>GSHMGKAAIGGPFSLIRDDGKRVTEKNLMGKWTILYFGFTHCPDICPDELIKLAAAIDKIKENSGVDVVPVFISVDPERDTVQQVHEYVKEFHPKLIGLTGSPEEIKSVARSYRVYYMKTEEEDSDYLVDHSIVMYLMSPEMNFVKFYGKNHDVDSLTDGV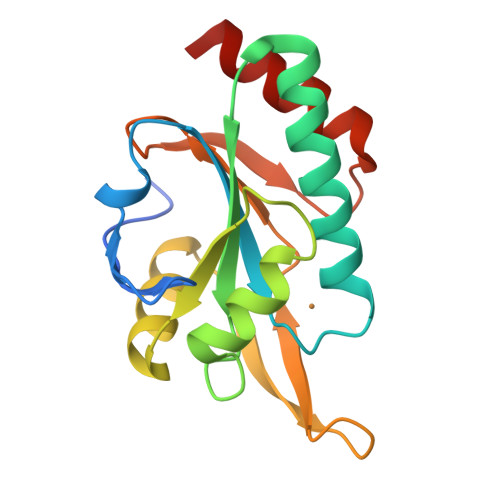VKEIRQYRK[3x]4-[(11S,15R)-4,4,7,7-Tetramethyl-16-oxatetracyclo[8.6.0.03,8.011,15]hexadeca-1(10),2,8-trien-11-yl]benzoic 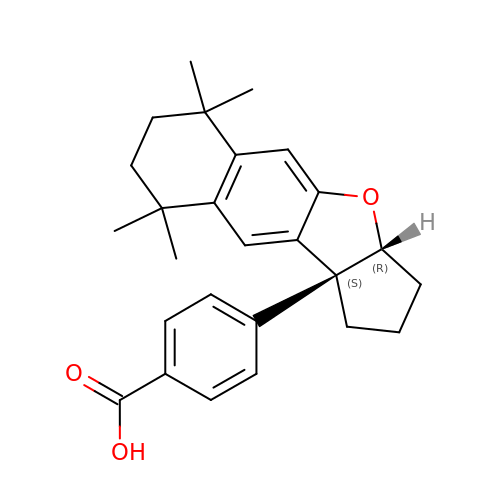acid | C26 H30 O3 | PLLRIXHLFVZTMU-GJZUVCINSA-N>[2x]GPMTLPKMEPSSHAPTEPDIQKDKDDSIIRENENIPAPLGTVVQLLFGSNTEYMQKVITRDKNNVNVETIPKFTPSLVEGGSRHYEYTKKLNNS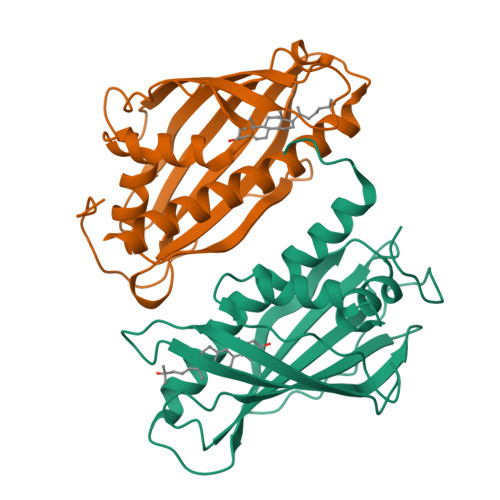IGPKQTKCLLTESIEHMDINNYVLVTQTTKTPDVPSGSNFAVESKIFLFWGQHDTTNMTVITKINWTSKSFLKGAIEKGSVEGQKVSVDYMLSELRDIISRAKSKKPVK> MGKMFFVDLSRCTACRGCQIACKQWKNLPAEETRNTGSHQNPPDLSYVTLKTVRFTEKSRKGPGIDWLFFPEQCRHCVEPPCKGQADVDLEGAVVKDETTGAVLFTELTAKVDGESVRSACPYDIPRID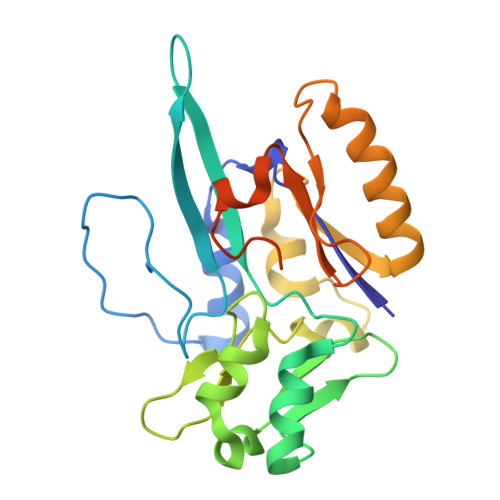PVTKRLSKCDMCNDRVQNGLLPACVKTCPTGTMNFGDEQEMLALAEKRLAEVKKTYPGAVLGDPNDVRVVYLFTRDPKDFYEHAVADLAPSMMTRQQLFARLFRPRA2-[4-(4-ethanoyl-3-ethyl-5-methyl-1~{H}-pyrrol-2-yl)-1,3-thiazol-2-yl]guanidine | C13 H17 N5 O 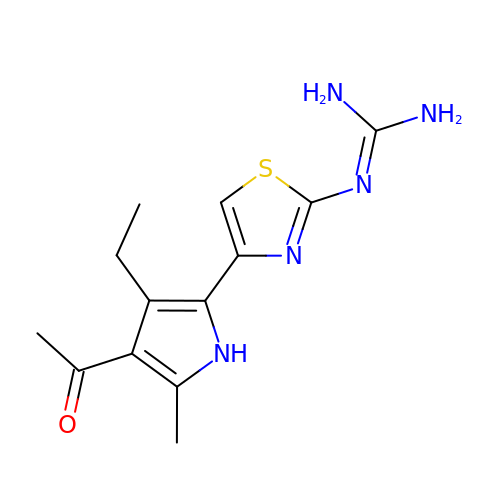S | RMIIUQZUCWLAPV-UHFFFAOYSA-N6-{[(4-nitrophenyl)methyl]sulfanyl}-9-beta-D-ribofuranosyl-9H-purine 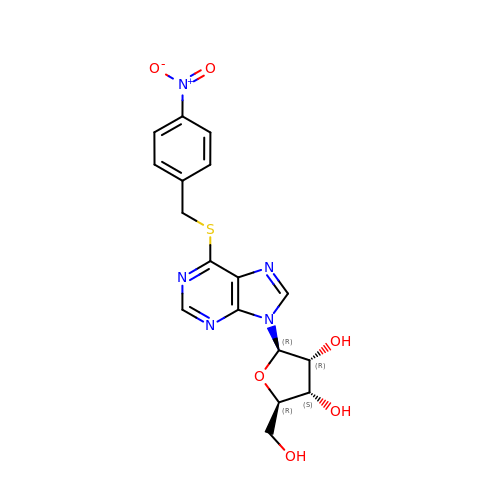| C17 H17 N5 O6 S | DYCJFJRCWPVDHY-LSCFUAHRSA-N4-(1-hydroxy-1,3-dihydrobenzo[c][1,2]oxaborole-6-carbonyl)-1,3,3-trimethylpiperazin-2-one | C15 H19 B N2 O4 | 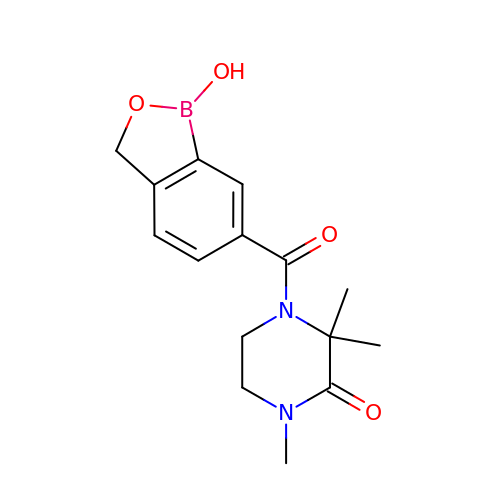BRKQWWXXHOEPIY-UHFFFAOYSA-N>[5x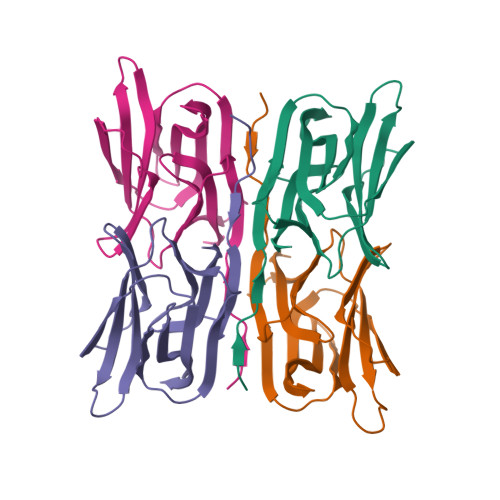]HHHHHHMALQLAAHSDARSGPVGSNGGQFWSFRPVRPLNKIVLSFSGSPDQTLNLISITFSSNPTDIITVGGVGPEPLTYTETVNIDGDIIEISGMIANYKGYNVIRSIKFTTNKKEYGPYGANAGTPFNIKIPDGNKIVGFFGNSGWYVDAIGAYYTAK>MNLKDSIGLRIKTERERQQMSREVLCLDGAELTVRQLIRIEKGESLPSLDRLSYIAKRLGKSMTELLDQDNITIPDEYYEMKNRLIKFPTYRNPDRIKSKLTLIEEVYEKFFDILPEEELLTLDILENILSFTSWEESPKVEEIYEDLFEQVKRKRKFSTNDLLVIDYYFFHLYGRKQY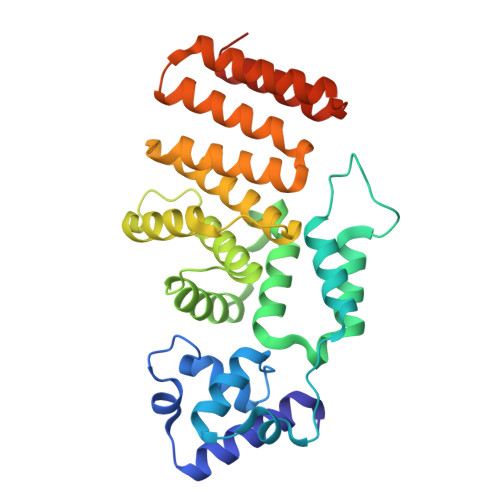DKKLFERIIKRVLNQEIWTDDVYNIVLFNDLMAIAALKIFHNSFSDFLTVVDKALAVIEKSQLYSYKPSVFVLKAKYELLHKENKKEAAENYDKAIVFASVLEDSVLEESIKAGKLADGLGAGWSHPQFEK[4x]> MPINIRRATINDIICMQNANLHNLPENYMMKYYMYH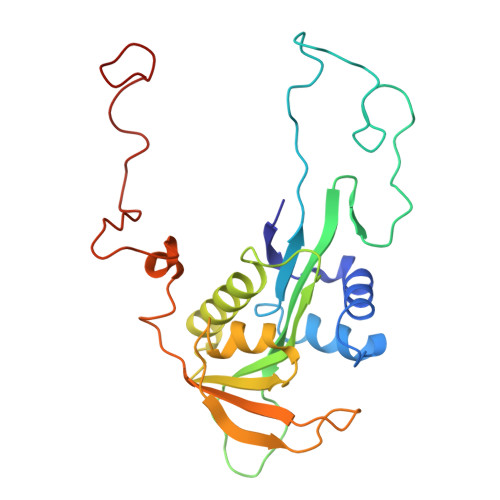ILSWPEASFVATTTTLDCEDSDEQDENDKLELTLDGTNDGRTIKLDPTYLAPGEKLVGYVLVKMNDDPDQQNEPPNGHITSLSVMRTYRRMGIAENLMRQALFALREVHQAEYVSLHVRQSNRAALHLYRDTLAFEVLSIEKSYYQDGEDAYAMKKVLKLEELQISNFTHRRLKENEEKLEDDLESDLLEDIIKQGVNDIIV Here, we present the near-atomic resolution structure of Haloferax tailed virus 1 (HFTV1), an archaeal virus thriving in extreme salinity. Through single-particle analysis, we obtained near-atomic resolution maps of DNA-filled and empty virions, enabling us to assemble full atomic models of the virus pre- and post-DNA release, including all structural protein components. The full atomic structure revealed that the virus has a length of 1350 Å and an icosahedral head with a diameter of ~600 Å. The tail has a length of 560 Å and terminates into a baseplate with three radiating TFs of ~190 Å in length.

The capsid forms a right-handed (dextro) icosahedron of a triangulation number T = 7 [h = 2, k = 1; (42, 43)], made up of 60 copies of the seven-protein asymmetric repeating unit. However, the handedness of HFTV1’s capsid is unusual, as most resolved structures of both tailed and untailed T = 7 icosahedral capsids display left-handed (levo) symmetry. The base layer of the capsid consists of gp19, the MCP. The MCP forms alternating pentamers and hexamers, which interact through asymmetric trimers. In each trimer, the MCPs adopt three distinct conformations. Lacking the first 100 amino acids, HFTV1 MCP fits the classical HK97 fold. The interior-facing surfaces of the MCP are highly negatively charged, which has been suggested to prevent the packaged DNA from sticking to the capsid, thus facilitating rapid release upon infection. The trimeric MCP interfaces are bound by trimers of gp18, the capsid stabilization protein (CSP). HFTV1 CSP binds the outer surface of each MCP trimer, thus stabilizing the capsid architecture. Each subunit in the MCP hexamer contains two intermolecular Mg2+ ions, as well as coordinating two additional Mg2+ ions in each subunit-subunit interface.

>[7x]MLMEAALPGSDVSAREVAKVWPGAKKGDYSFLQGNQSRSLEAEMTRTARAEAGTDRHRALKDYAVDADNLPKTLSAGSKHLTEDGDVIEARLDDAIPRMLFAASDPEYVDTLFREQLLEVVMEGRELRKVAREASNVINANTRVGDVPIASDEEFARPTGQGAEIRDDGETYTTVAWNATKLTEGSRVTDEMRDQAMVDLIERNIQRVGASLENGINRVFLTELVDNAQNNHDTAGSNQGYQALNSAVGEVDKDDFRPDTYVTHPDYRTQLFNDTNLAYANRAGTNEVLRNREDAPIVGDIAGLDMHAAMSSATYDDGTDIGWSGGSETWGFSSDGDKGAVVYDRDNIHTILYAPNGQDVEIKDYEDPIRDITGVNGRLHVDCQYSQGRSSATVQY;>MATETQGEHTFPVEVLISGEELRGYTAGEALSAGEPVYLSGDYEVSASSADGGEFLGVNLYDVASGEPVALAGDDCEVRVEVSEQVTANDEILPDGLGTFETVATSAASAGVAIVQEGAASGEVCEAYIFAVQGTTA[7x];>MTDTIVNVQGSFFSASASGVADTESLLIDPQDAKFGAIEIHNIAHGGSVDVELLTSSDDTELVEDAAVTLDSFTGEGISQGNQIEASDNTNTYIRITNTSGGAIDIIATGREVSQ[6x]>[3x]GSPIGIPMSGQSLTDRITAAQHSVTGSAVSKTVCKATTHEIMGPKKKHLDYLIQCTNEMNVNIPQLADSLFERTTNSSWVVVFKSLITTHHLMVYGNERFIQYLASRNTLFNLSNFLDKSGLQGYDMSTFIRRYSRYLNEKAVSYRQVAFDFTKVKRGADGVMRTMNTEKLLKTVPIIQNQMDALLDFNVNSNELTNGVINAAFMLLFKDAIRLFAAYNEGIINLLEKYFDMKKNQCKEGLDIYKKFLTRMTRISEFLKVAEQVGIDRGDISGSGSGHMDRVRNLQSEVEGVKNIMTQNVERILARGENL

Here, we show that the R-SNAREs VAMP8, VAMP3, and VAMP2, which cycle between the plasma membrane and endosomes, bind directly to the ubiquitously expressed, PtdIns4,5P2-binding, endocytic clathrin adaptor CALM/PICALM. X-ray crystallography shows that the N-terminal halves of their SNARE motifs bind the CALMANTH domain as helices in a manner that mimics SNARE complex formation. In this study, we provide structural, biochemical and in vivo data to show that the internalization of VAMP8, and consequently that of the highly related small R-SNAREs, VAMP3 and VAMP2, is mediated by specific, direct interactions between the N-terminal halves of their SNARE motifs and the ANTH (AP180 N-terminal Homology) domain of the endocytic clathrin adaptor CALM. Thus, CALM:R-SNARE interactions ensure that R-SNAREs, required for the fusion of endocytic clathrin-coated vesicles with endosomes and also for subsequent postendosomal trafficking, are sorted into endocytic vesicles.

In an attempt to obtain a structure of a complex between CALMANTH and VAMP8, a construct was designed in which residues 11–41 of VAMP8 were fused through an artificial linker of six residues to residues 1–264 of CALMANTH. The resulting chimeric protein (CALMANTH(1-264):VAMP8(11-41)) crystallized and its 2.0 Å resolution structure (final R/Rfree 0.183/0.199) showed unambiguously that residues 15–38 of VAMP8 form a single α helix with residues between Phe16 and Arg37 contacting CALMANTH, consistent with the truncation data. The VAMP8 helix fitted into the spatially complementary groove of CALMANTH, lined by residues from helix 9 and helix 10, which was blocked by helix 11 in the unliganded CALMANTH structures and by dimerization in CALMANTH(1-264). There was a small movement of helices 9 and 10 with respect to each other that caused a slight widening of the groove as compared with the unliganded domain structure. No electron density was visible for 17 residues that connect the last ordered residue of CALM with the first of VAMP8. This would allow considerable flexibility in the positioning of the VAMP8 and indeed in the crystals where it bound to CALMANTH a VAMP8 SNARE motif could reach an adjacent ANTH domain to which it was not covalently linked. Key residues in the interaction, 13 on VAMP8 and 16 on CALM, are spread throughout the interface between the two proteins. The residues in the CALMANTH:VAMP8 interface are highly conserved from human to fish. The interface is mainly hydrophobic in nature, burying a total of 1500Å2 of accessible surface area, and a full list of interacting residues is given in Figure 5D. The residues Lys24 and Met27 of VAMP8 play key roles in the interaction, explaining their initial identification as residues of importance for VAMP endocytosis (Grote et al., 1995) (Lewis et al., 2000).> MERRLIFGTIASKMSLAP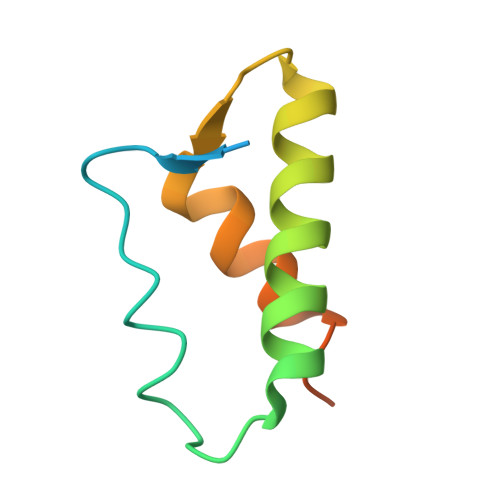EADLDSLIIRNDSLSGAVIAAIMQEAGLRAVRKNRYVILQSDLEEAYATQVKTDNTVDKFDFYK>[6x]GPLGSMAESEDRSLRIVLVGKTGSGKSATANTILGEEIFDSRIAAQAVTKNCQKASREWQGRDLLVVDTPGLFDTKESLDTTCKEISRCIISSCPGPHAIVLVLQLGRYTEEEQKTVALIKAVFGKSAMKHMVILFTRKEELEGQSFHDFI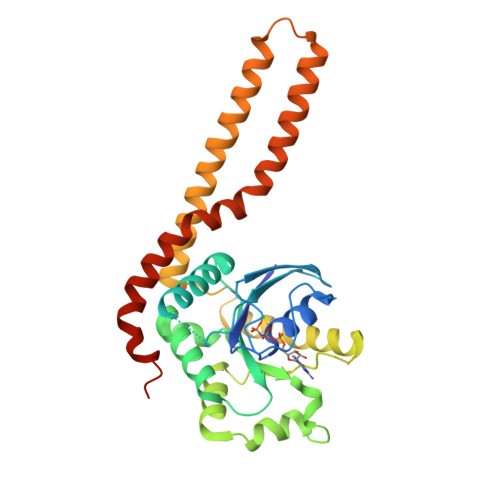ADADVGLKSIVKECGNRCCAFSNSKKTSKAEKESQVQELVELIEKMVQCNEGAYFSDDIYKDTEERLKQREEVLRKIYTDQLNEEIKLVEEDKHKSEEEKEKEIKLLKLKYDEKIKNIREEAERNIFKDVFNRIWKMLSEIWHRFLSKCKFYSS>ALVPMVIEQTSRGERSFDIYSRLLKERVIFLTGQVEDHMANLIVAQMLFLEAENPEKDIYLYINSPGGVITAGMSIYDTMQFIKPDVSTICMGQAAS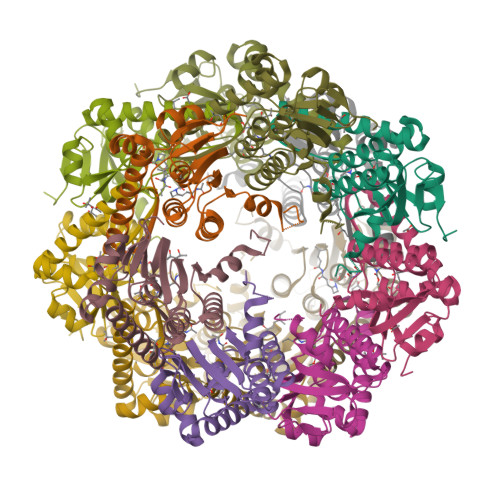MGAFLLTAGAKGKRFCLPNSRVMIHQPLGGYQGQATDIEIHAREILKVKGRMNELMALHTGQSLEQIERDTERDRFLSAPEAVEYGLVDSILTHRN[28x]> AAAGGTGGAAAGAACTCAAGAGAAGTGTACTGTCATTTTTAGATTAAGAGGA;> TTGGTGGTGGATGTTAGCAAACGCGTCGAGAGCCACCCTTGAAAAGGTTAAGCAA;> AATAACGGCTCAGAGC;> TTGGTGGTGGGAAAATTCATATGGTAACACTAAAGTTTTGAAGCCTTAAGATTCAAAAG;> AGAAACGCAAAGGCGACATGGGATAGCTGAATTTTAAACATTAGTCAAATC;> TTGGTGGAAAGGTGAATTATCACACGGAAATTATTCATTAAAACAG;> TCAACCGAGCTTGCTT;> AAATATTGCGTCACCGTGATACCGTCGTCACCATCAACATCGTAACCG;> TTGGTGGTGGTGGTGCGGAAACGTCACCAATTTACCATTCGAAAGAG;> TATTAGCGAGATGGTTTTATTACA;> TTGGTGGTGGTGGTGCGGCATTTACCGCCTCCCTAAAAAAAAACAG;> CGACAGAATGAAAGAG;> CGTCAGACAGCCCCCTGGCGCATAGCCCTGAC;> ACCGCCACCAGAGCCAGAACAACATAATTTCATCCAACGT;> TTGGTGGTGGTGCAGAGCCGCCACTTATTACGCAGTAAAAAAACAG;> CATAATCAAAATCACCGGAACCCTCAGAGACCAGAGC;> CCACCGGATCGGTCATTGTAGCGCGTCAATCATACAACGGATCCCCGG;> GTAAGCGTTTTAGACTATTATAGTCAGAAGCAAAGCG;> CGCCACCAGATTCATC;> GAGGCAGGTGGAAAGCCGTCATAACATAAATCAAAAATCA;> CCCTGCCTATTTCCTGGAAGTTTCAT;> TGATGATACAGGAGGATTAGGGCTTAATTAATGGTCAATA;> CCCGTATACTCATTAAAGCCAGAATCAGACGAAGACGACGATTACGAG;> CACCCTCATGTTTAGCATCGGTTGTAC;> CGTACTCAGGAGGTAGCATTAACATC;> ATAAGTGCTAGAAAATTTTATTTTGTCACAATCAATAAAAAAAACAG;> GGGTTGATGAACGAGTAAATATGCAACTAAAG;> TTAGTAAAAAGCCCAAAAAGCTAATATATTTTCATTTGGG;> GTTAGCGTAATAGAAAGGAACAACTGAAAATCTATTTAAA;> ATTCCACAGACAGTTTAGAACCCTCA;> CATGTACCGTTTACCATTTCAACAGCCTTTAAAGCCCCAA;> TTGTATCGAAACAGCTACTTGAGCTAGCACCAGAAACCATAAACAAAG;> CAAAAGGAGTTTCAGCATCGATGAATAAATTAATGCCGGATGTAGGTA;> AATAATTTTTTCACGTTAAAGGAATCATTGCCGAGAGATCTACAAAGG;> CGAAAGACATCACCAGCATTTGGGAATTAGAG;> TTGCGGGAATAGTTGCTTTTTTAAAAACAGGAAGATTGTA;> TATTCGGTCGCTGAGGCCACGCATAATTCGCATTGTAAACGTTAATAT;> TCGAGGTGATTCGCGT;> AATTTCTTGTTTATCATTGAGGGAGACAAAAGGACACCACAGAGCCACGCTCAGTA;> TGACAACAACCATCGCCTTGCAGGTCGGATTCGGGATAGG;> AGGCACCAATCATCGCCTGATAAACTTAGCCGGAAGCATA;> GTAAAATACGTAATGCAGTTTCCACCATTCGCTGGTGCCGGAAACCAG;> GGCTTTGAAAGGGCGATCGCACTCCAGCCAGC;> ACCAACTTTCAAGTTTGCACCGTAATCAGTAG;> TAAGGGAATCCGCTCACCGCTTTCCAGTCGGG;> GACCTGCTCCATGTTATTGTGTCGAAGCTTGCCGTTGTAAAACGACGG;> CCCCCAGCTGGTCATA;> TAAGGCTTGGCTGGCTCTCACTGCCAATTCCACACAACAT;> GACAGATGCGTGCCAG;> CAAGAACCTGAGTGAGAAGTGTAAAGCCTGGG;> GGTAGAAAGAACCACCCCACCACCAATACCCACAACATATGGGGTTTT;> TAAATTGGGCTTGTTTGCCATCTTTT;> ATTACCTTCTACGTTACAAAAGGAATAAAAAC;> TTTTGCAATCAACTAATGCAGATAACGTGGACACTTTAAT;> CAAAATAGTGCGGAATGCAGTCTCGGGTCAGTAAGTATTACATGTTTT;> CGTTTACCTTGGCCTTCGTTGGGAAGAAAAATATGCGATT;> ATCATAACCCTCCTCAAATAATAAATCAACAGTTAATGCC;> AGTTGAGAGTCTATCA;> TACCACATAAGAAGTTTTGCCAGAGGGGG;> CATAACGCATAAAACGAGGAGGTT;> GCATAGTATCCAGTTTTTAAGAACAATCAACG;> TTAAACAGTTCGCGAACCAGACCG;> AATCTTGATAACAAAGGGGTGGTTATTGCCCTTCAC;> TAATAGTAAAATGCATACATGGCTTT;> GGATAGCGTCCAATACCGAGAGGCGCATTGACAACTAACG;> GAGTACCTTCGCGTTTTAATTCGAGCTTCAAAAGAAAACG;> GGATTAGATAACAGTGAGAATGACATATTCATTGAATCCC;> GAAGCAAACTCCAACAGGTCATACGGTGTGGAACCTAAGCCCGGAATAGGTGTATCAC;> GATTGCATCAAAAGCGGATGGCTT;> AGCCCGAAAGACGGTCTTTATTTTAACGTGAATTTATAAGACTCCCCTCAGA;> TTCAAATATTAATTGCTCCTTTTGTAGCTCAAAGAGGCTG;> ATTTCGCAGCTGAATATAATGCTGATAAGAGGGTAATAAGCCCTGACT;> TTAGATACCCAGGCGGAGACTCCTGGCATGATCCGTTCCACGCCGCCA;> AGATTTAGTTTGACCAGCGCGAGCCAGAACCG;> AATTCTGCATAAGTATTTATTCTGAAACATGAGCCTTGAG;> TCCATATAACAGTTGATTCCCAATAGTAGTTTAGTACACAAACTACAACGCCTGTAGC;> TAAAGCCTTTGCGGGAGTCGTCTTTCTAGCTGACGGTAATCGTAAAACATCAGAAA;> CAATAAATCATACAGGCAAGGTAAAAATTCCCTCATACTATTTTT;> GGTGAGAAAGGCTCAACCGTTCCAGACGTAAACAACGCGCCAAAGGGAAGGT;> TATATTTTAAATGCAATGCCTGAGTAATGGAGGGTAG;> TAATACTTCAGAGCATTAGGAACCCCACCCTCGGAATAAGACATACAT;> TATTTCAACGCAAGGACAAAGAATTCACCAGTCGCCACCCTCAGAACC;> ACAAGAGAGGAGTGAGAACGATCTGAGTTTCGTAGCAAAATGGCATCAATTCTACT;> TGAGAGTCTGGAGCAATAAGCAAATCCAAAAA;> CTATCAGGTTGCGAAT;> ACCATCAATATGATATCGGAGACATGACCCTG;> CCAATAGGAACGCCATCAGCTTTCCTCAGCAGGCTACAGAGCAAAAGA;> TTAAATTTTTGTTAAAACAACCCGGAGTTAAACATGAGGACACTACGA;> TTTGTTAAAACCGATA;> TGTACCCCGGTTGATATAGCATGTGATTTTGC;> TGCATCTGCAGGAAGATCGGTGCGGGCCTCTT;> TCACGTTGACCGCTTCCATTCAGGCTGCGCAAGTTTTCCC;> CTGGCCTTCCTGTAGCCAAAAATA;> AGCGAGTATCAGCTCAGCCGACAAAAAGGCTC;> GCAAAGCGTTAAACGGACCGTAATTCCGTGGGAACAAACG;> ACGACAGTATCGGCCTCCAGTTTGTAGCAACG;> TTTCCGGCGTGTAGATGACTTTTTGGCCGCTT;> TCTAGAGGAGATTTGTACCTAAAAAGCAAGGCAAAAAAAAAAAACAG;> CCAGTGCCAAATCCGC;> GGCGAAAGGGGGATGTCGCTATTAAACGAGGGAGGGGACG;> GCTGCAAGATACACTACAAGCGCGCGATAGCAGCCTTTAG;> GCGATTAAGTACCGAGCTCGAATTAATTGTTACCGAACTGACAGACCA;> GTTGGGTAACGCCAGGCTGTTGGGGGACTAAAGGGCGCATTAAATGTG;> AGTCACGAATGCCTGCAGGTCGACACGAGCCGGAACGAGGTCAAGAGT;> CTAACTCACATTAATTGGGCGCCACTGCTCATTCCCTTATAGTCCACTATTAAAGA;> GTGCCTAAGGATATTC;> GCTGTTTCCTGTGTGACGTAATCAGATTATACAAACACTCCCAGCAAAAGCATCGG;> CGCCTGGCCCTGCGGCAAAATCAGTGAACATTGTGA;> AGACGGGCCCGAGATAATTACCCATGGCTCATTAT;> GCCAACGCGAGAAACACCTGTTTGCAAAGGGCGAAAAACCTTTAGGAA;> GCGGGGAGGCAGCAAGCGGTCCACGCTGGTTTGCCCC;> TGCGTATTGCGTTGCGGACCTTCACGCAGACGGTTTTCATAAAAAAAAAAAACAG;> TGATAGACGGTTTTTCGCCCTTTGACGTTGGAGTCCACGTTCTTTAATAGTGGACTCTTGTTCCAAACTGGAACAACACTCAAAAATATCTCGGGCTATTCTTTTGATTTATAAGGGATTTTGCCGATTTCGGAACCACCATCAAACAGGATTTTCGCCTGCTGGGGCAAACCAGCGTGGACCGCTTGCTGCAACTCTCTCAGGGCCAGGCGGTGAAGGGCAATCAGCTGTTGCCCGTCTCACTGGTGAAAAGAAAAACCACCCTGGCGCCCAATACGCAAACCGCCTCTCCCCGCGCGTTGGCCGATTCATTAATGCAGCTGGCACGACAGGTTTCCCGACTGGAAAGCGGGCAGTGAGCGCAACGCAATTAATGTGAGTTAGCTCACTCATTAGGCACCCCAGGCTTTACACTTTATGCTTCCGGCTCGTATGTTGTGTGGAATTGTGAGCGGATAACAATTTCACACAGGAAACAGCTATGACCATGATTACGAATTCGAGCTCGGTACCCGGGGATCCTCTAGAGTCGACCTGCAGGCATGCAAGCTTGGCACTGGCCGTCGTTTTACAACGTCGTGACTGGGAAAACCCTGGCGTTACCCAACTTAATCGCCTTGCAGCACATCCCCCTTTCGCCTAATAGCGAAGAGGCCCGCACCGATCGCCCTTCCCAACAGTTGCGCAGCCTGAATGGCGAATGGCGCTTTGCCTGGTTTCCGGCACCAGAAGCGGTGCCGGAAAGCTGGCTGGAGTGCGATCTTCCTGAGGCCGATACTGTCGTCGTCCCCTCAAACTGGCAGATGCACGGTTACGATGCGCCCATCTACACCAACGTGACCTATCCCATTACGGTCGTTTGTTCCCACGGAGAATCCGACGGGTTGTTACTCGCTCACATTTAATGTTGATGAAAGCTGGCTACAGGAAGGCCAGACGCGAATTATTTTTGATGGCGTTCCTATTGGTTAAAAAATGAGCTGATTTAACAAAAATTTAATGCGAATTTTAACAAAATATTAACGTTTACAATTTAAATATTTGCTTATACAATCTTCCTGTTTTTGGGGCTTTTCTGATTATCAACCGGGGTACAACATGCTAGTTTTACGATTACCGTTCATCGATTCTCTTGTTTGCTCCAGACTCTCAGGCAATGACCTGATAGCCTTTGTAGATCTCTCAAAAATAGCTACCCTCTCCGGCATTAATTTATCAGCTAGAACGGTTGAATATCATATTGATGGTGATTTGACTGTCTCCGGCCTTTCTCACCCTTTTGAATCTTTACCTACACATTACTCAGGCATTGCATTTAAAATATATGAGGGTTCTAAAAATTTTTATCCTTGCGTTGAAATAAAGGCTTCTCCCGCAAAAGTATTACAGGGTCATAATGTTTAAAGTACAACCGATTTAGCTTTATGCTCTGAGGCTTTATTGCTTAATTTTGCTAATTCTTTGCCTTGCCTGTATGATTTATTGGATGTTAATGCTACTACTATTAGTAGAATTGATGCCACCTTTTCAGCTCGCGCCCCAAATGAAAATATAGCTAAACAAAATATTGACCATTTGCGAAATGTATCTAATGGTCAAACTAAATCTACTCGTTCGCAGAATTGGGAATCAACTGTTATATGGAATGAAACTTCCAGACACCGTACTTTAGTTGCATATTTAAAACATGTTGAGCTACAGCATTATATTCAGCAATTAAGCAAAAAGCCATCCGCAAAAATGACCTCTTATCAAAAGGAGCAATTAAAGGTACTCTCTAATCCTGACCTGTTGGAGTTTGCTTCCGGTCTGGTTCGCTTTGAAGCTCGAATTAAAACGCGATATTTGAAGTCTTTCGGGCTTCCTCTTAATCTTTTTGATGCAATCCGCTTTGCTTCTGACTATAATAGTCAGGGTAAAGACCTGATTTTTGATTTATGGTCATTCTCGTTTTCTGAACTGTTTAAAAAATTTGAGGGGGATTCAATGAATATTTATGACGATTCCGCAGTATTGGACGCTATCCAGTCTAAACATTTTACTATTACCCCCTCTGGCAAAACTTCTTTTGCAAAAGCCTCTCGCTATTTTGGTTTTTATCGTCGTCTGGTAAACGAGGGTTATGATAAAGTTGCTCTTACTATGCCTCGTAATTCCTTTTGGCGTTATGTATCTGCATTAGTTGAATGTGGTATTCCTAAATCTCAACTGATGAATCTTTCTACCTGTAATAATGTTGTTCCGTTAGTTCGTTTTATTAACGTAGATTTTTCTTCCCAACGTCCTGACTAAAATAATGAGCCAGTTCTTAAAATCGCATAAGGTAATTCACAATGATTAAAGTTGAAATTAAACCATCTCAAGCCCAATTTACTACTCGTTCTGGTGTTTCTCGTCAGGGCAAGCCTTATTCACTGAATGAGCAGCTTTGTTACGTTGATTTGGGTAATGAATATCCGGTTCTTGTCAAGATTACTCTTGATGAAGGTCAGCCAGCCTATGCGCCTGGTCTGTACACCGTTCATCTGTCCTCTTTCAAAGTTGGTCAGTTCGGTTCCCTTATGATTGACCGTCTGCGCCTCGTTCCGGCTAAGTAACATGGAGCAGGTCGCGGATTTCGACACAATTTATCAGGCGATGATACAAATCTCCGTTGTACTTTGTTTCGCGCTTGGTATAATCGCTGGGGGGAGTGTTTTAGTGTATTCTTTTGCCTCTTTCGTTTTAGGTTGGTGCCTTCGTAGTGGCATTACGTATTTTACCCGTTTAATGGAAACTTCCTCATGAAAAAGTCTTTAGTCCTCAAAGCCTCTGTAGCCGTTGCTACCCTCGTTCCGATGCTGTCTTTCGCTGCTGAGGGTGACGATCCCGCAAAAGCGGCCTTTAACTCCCTGCAAGCCTCAGCGACCGAATATATCGGTTATGCGTGGGCGATGGTTGTTGTCATTGTCGGCGCAACTATCGGTATCAAGCTGTTTAAGAAATTCACCTCGAAAGCAAGCTGATAAACCGATACAATTAAAGGCTCCTTTTGGAGCCTTTTTTTTGGAGATTTTCAACGTGAAAAAATTATTATTCGCAATTCCTTTAGTTGTTCCTTTCTATTCTCACTCCGCTGAAACTGTTGAAAGTTGTTTAGCAAAATCAAAATTCATTTACTAACGTCTGGAAAGACGACAAAACTTTAGATCGTTACGCTAACTATGAGGGCTGTCTGTGGAATGCTACAGGCGTTGTAGTTTGTACTGGTGACGAAACTCAGTGTTACGGTACATGGGTTCCTATTGGGCTTGCTATCCCTGAGGGTGGTGGCTCTGAGGGTGGCGGTTCTGAGGGTGGCGGTTCTGAGGGTGGCGGTACTAAACCTCCTGAGTACGGTGATACACCTATTCCGGGCTATACTTATATCAACCCTCTCGACGGCACTTATCCGCCTGGTACTGAGCAAAACCCCCCTAATCCTTCTCTTGAGGAGTCTCAGCCTCTTAATACTTTCATGTTTCAGAATAATAGGTTCCGAAATAGGCAGGGGGCATTAACTGTTTATACGGGCACTGTTACTCAAGGCACTGACCCCGTTAAAACTTATTACCAGTACACTCCTGTATCATCAAAAGCCATGTATGACGCTTACTGGAACGGTAAATTCAGAGACTGCGCTTTCCATTCTGGCTTTAATGAGGATTTATTAAATTGTGAATATCAAGGCCAATCGTCTGACCTGCCTCAACCTCCTGTCAATGCTGGCGGCGGCTCTGGTGGTGGTTCTGGTGGCGGCTCTGAGGGTGGTGGCTCTGAGGGTGGCGGTTCTGAGGGTGGCGGCTCTGAGGGAGGCGGTTCCGGTGGTGGCTCTGGTTCCGGTGATTTTGATTATGAAAAGATGGCAAACGCTAATAAGGGGGCTATGACCGAAAATGCCGATGAAAACGCGCTACAGTCTGACGCTAAAGGCAAACTTGATTCTGTCGCTACTGATTACGGTGCTGCTATCGATGGTTTCATTGGTGACGTTTCCGGCCTTGCTAATGGTAATGGTGCTACTGGTGATTTTGCTGGCTCTAATTCCCAAATGGCTCAAGTCGGTGACGGTGATAATTCACCTTTAATGAATAATTTCCGTCAATATTTACCTTCCCTCCCTCAATCGGTTGAATGTCGCCCTTTTGTCTTTGGCGCTGGTAAACCATATGAATTTTCTATTGATTGTGACAAAATAAACTTATTCCGTGGTGTCTTTGCGTTTCTAAAATATGTTGCCACCTTTATGTATGTATTTTCTACGTTTGCTAACATACTGCGTAATAAGGAGTCTTAATCATGCCAGTTCTTTTGGGTATTCCGTTATT;> GGAACAAGAAATCAAAAGAATAGCAACAGCTGTTTCTTTTCACC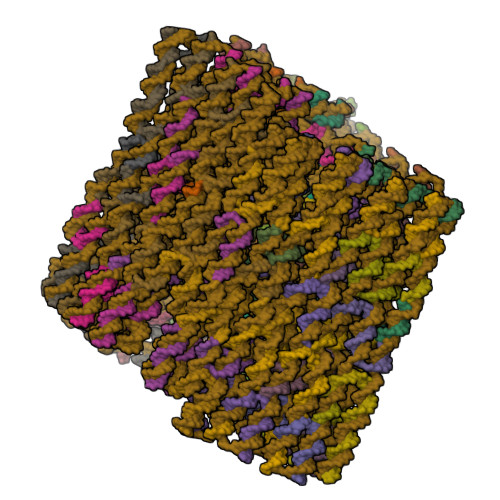AGTG;> TTGAGTGTTGTAGAGCAACAGTCAGGAGATATTCACAA;> AGCAGGCGAAAATCCAGAACGAGTAG;> ATGGTGGTTCCGAAATAGAGAGTTAGGCGGTT;> CTGCATTAATGAATCGAAACCTGTAACGGTGT> GPLGSNSF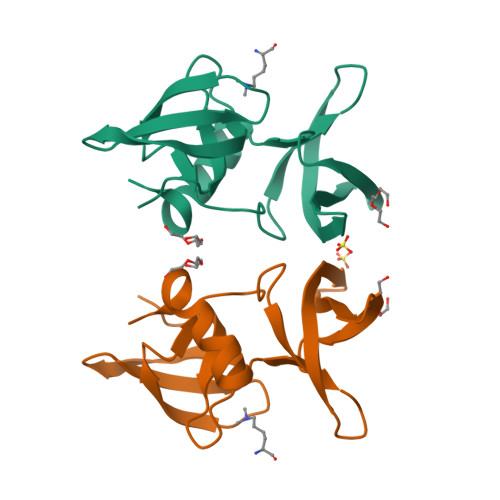VGLRVVAKWSSNGYFYSGKITRDVGAGKYKLLFDDGYECDVLGKDILLCDPIPLDTEVTALSEDEYFSAGVVKGHRKESGELYYSIEKEGQRKWYKRMAVILSLEQGNRLREQYGLG;> SSHLKSKKGQ1-({5-[4-(methylsulfonyl)phenoxy]-2-pyridin-2-yl-1H-benzimidazol-6-yl}methyl)pyrrolidine-2,5-dione | C24 H20 N4 O5 S 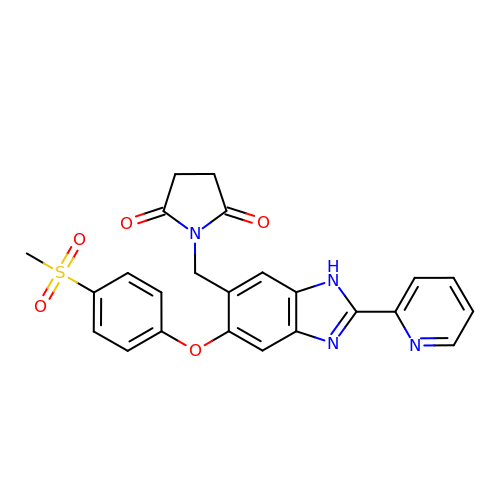| IPZLCOKXDRIZBC-UHFFFAOYSA-N>MTASAPDGRPGQPEATNRRSQLKSDRRFQLLAAAERLFAERGFLAVRLEDIGAAAGVSGPAIYRHFPNKESLLVELLVGVSARLLAGARDVTTRSANLAAALDGLIEFHLDFALGEADLIRIQDRDLAHLPAVAERQVRKAQRQYVEVWVGVLRELNPGLAEADARLMAHAVFGLLNSTPHSMKAADSKPARTVRARAVLRAMTVAALSAADRC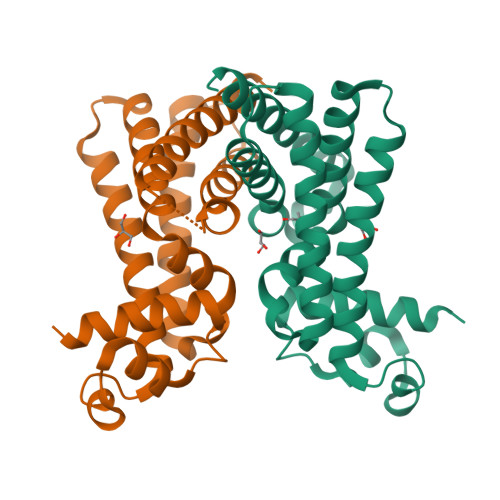L[4x]> LPDSVDWREKGCVTEVKYQGSCGACWAFSAV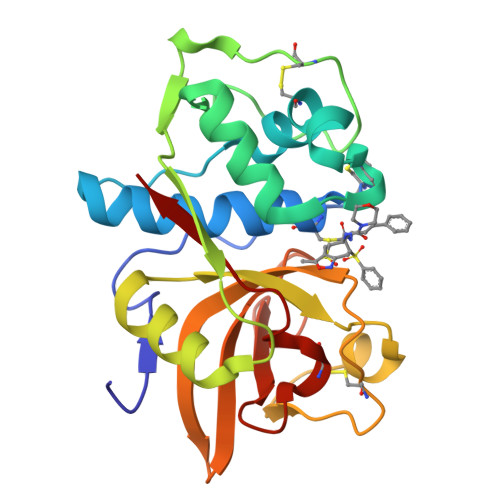GALEAQLKLKTGKLVSLSAQNLVDCSTKKYGNKGCNGGFMTTAFQYIIDNKGIDSDASYPYKAMDQKCQYDSAYRAATCRKYTELPYGREDVLKEAVANKGPVSVGVDARHPSFFLYRSGVYYEPSCTQNVNHGVLVVGYGDLNGKEYWLVKNSWGHNFGEKGYIRMARNKGNHCGIASFPSYPEI>[2x]MASWSHPQFEKGASTSLYKKAGRMSKFTWKELIQLGSPSKAYESSLACIAHIDMNAFFAQVEQMRCGLSKEDPVVCVQWNSIIAVSYAARKYGISRMDTIQEALKKCSNLIPIHTAVFKKGEDFWQYHDGCGSWVQDPAKQISVEDHKVSLEPYRRESRKALKIFKSACDLVERASIDEVFLDLGRICFNMLMFDNEYELTGDLKLKDALSNIREAFIGGNYDINSHLPLIPEKIKSLKFEGDVFNPEGRDLITDWDDVILALGSQVCKGIRDSIKDILGYTTSCGLSSTKNVCKLASNYKKPDAQTIVKNDCLLDFLDCGKFEITSFWTLGGVLGKELIDVLDLPHENSIKHIRETWPDNAGQLKEFLDAKVKQSDYDRSTSNIDPLKTADLAEKLFKLSRG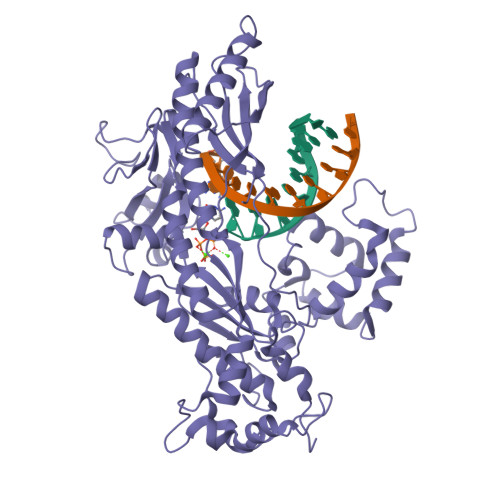RYGLPLSSRPVVKSMMSNKNLRGKSCNSIVDCISWLEVFCAELTSRIQDLEQEYNKIVIPRTVSISLKTKSYEVYRKSGPVAYKGINFQSHELLKVGIKFVTDLDIKGKNKSYYPLTKLSMTITNFDIIDLQKTVVDMFGNQVHTFKSSAG>MGGSTKLEEHLEGIVNIFHQYSVRKGHFDTLSKGELKQLLTKELANTIKNIKDKAVIDEIFQGLDANQDEQVDFQEF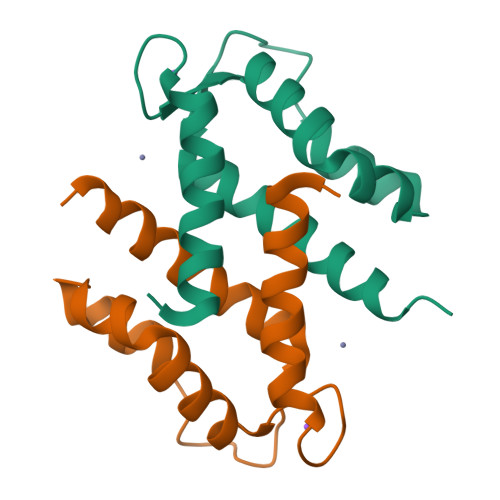ISLVAIALKAAHYHTHKE[2x]2-(4-{[3-(piperidin-1-yl)propyl]amino}quinolin-2-yl)benzonitrile 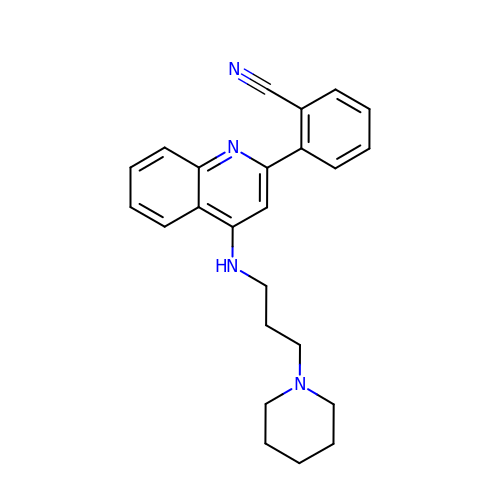| C24 H26 N4 | PBIFICWHSUFSCR-UHFFFAOYSA-N> MAASSRAQVLALYRAMLRESKRFSAYNYRTYAVRRIRDAF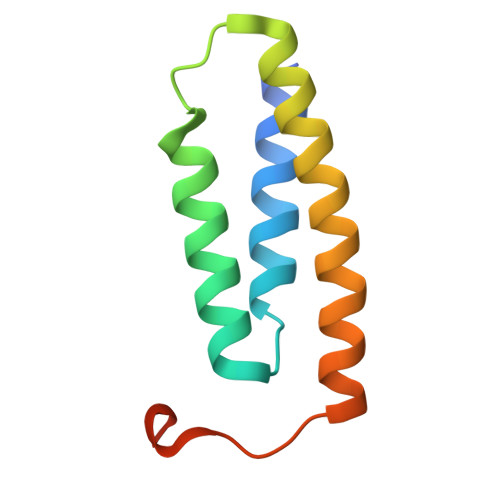RENKNVKDPVEIQTLVNKAKRDLGVIRRQVHIGQLYSTDKLIIENRDMPRT>[2x]MMLPKDFQWGFATAAYQIEGAIDKDGRGPSIWDTFCAIPGKIADGTSGVTACDSYNRTAEDIALLKSLGAKSYRFSISWSRIIPKGGRDDPVNQLGIDHYAQFVDDLLEAGITPFITLFHWDLPEELHQRYGGLLNRTEFPLDFENYARVMFKALPKVRNWITFNEPLCSAIPGYGSGTFAPGRQSTTEPWIVGHNLLVAHGRAVKVYRDEFKDLNDGQIGIVLNGDFTYPWDSSDPLDREAAERRLEF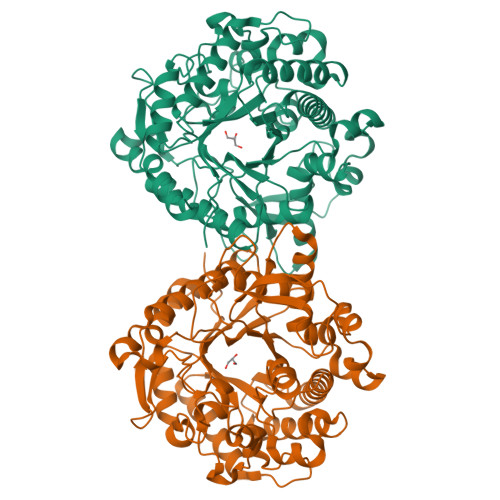FTAWYADPIYLGDYPASMRKQLGDRLPEFTPEEKAFVLGSNDFYGMNHYTSNYIRHRTSPATADDTVGNVDVLFYNKEGQCIGPETESSWLRPCPAGFRDFLVWISKRYNYPKIYVTENGTSLKGENDLPKEKILEDDFRVNYYNEYIRAMFTAATLDGVNVKGYFAWSLMDNFEWADGYVTRFGVTYVDYENGQQRFPKKSAKSLKPLFDELIAKE> MGRVYYGGVERTYLYRGRILNLALEGRYEIVEHKPAVAVIALREGRMLFVRQMRPAVGLAPLEIPAGLIEPGEDPLEAARRQLAEETGLSGDLTYLFSYFV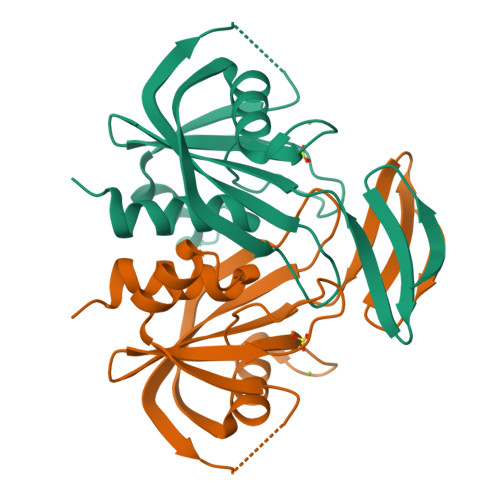SPGFTDEKTHVFLAENLKEVEAHPDEDEAIEVVWMRPEEALERHQRGEVEFSATGLVGVLYYHAFLRGR> GGSMADKEKAEGNKFYKARQFDEAIEHYNKAWELHKDITYLNNRAAAEYEKGEYETAISTLNDAVEQGREMRADYKVISKSFARIGNAYHKLGDLKKTIEYYQKSLTEHRTADILT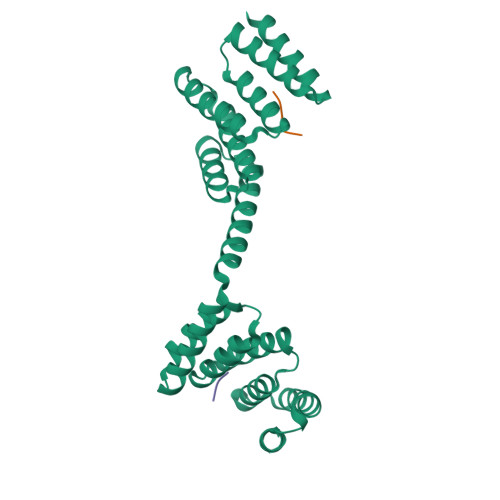KLRNAEKELKKAEAEAYVNPEKAEEARLEGKEYFTKSDWPNAVKAYTEMIKRAPEDARGYSNRAAALAKLMSFPEAIADCNKAIEKDPNFVRAYIRKATAQIAVKEYASALETLDAARTKDAEVNNGSSAREIDQLYYKASQ;>MEEVD[2x]> MQDAITAVINNYDVQGKYLDGAALDKLKAYFTTGAVRVRAAAVISSNATT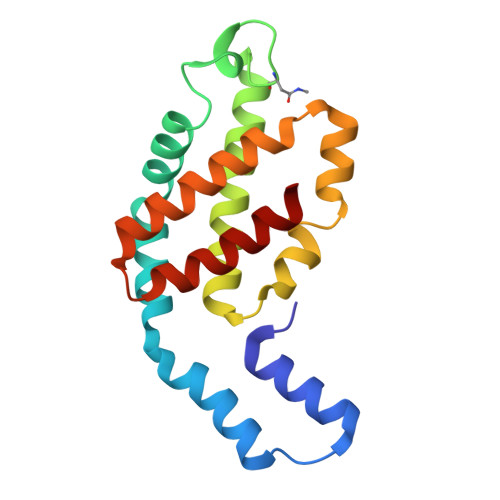IIKEAAAKALIYSDLTRPGGNMYTTRRYAACIRDMDYFLRYATYAMLAGDPSILDERVLNGLKETYNSLGVPIAATVGGIQAMKEVVGGLVGPDAAKEASIYFDYLSSGLS>MCWAAAIPIAISGAQAISGQNAQAKMIAAQTAAGRRQAMEIMRQTNIQNADLSLQARSKLEEASAELTSQNMQKVQAIGSIRAAIGESMLEGSSMDRIKRVTEGQFIREANMVTENYRRDYQAIFAQQLGGTQSAASQIDEIYKSEQKQKSKLQMVLDPLAIMGSSAASAYASGAFDSKSTTKAPIVAAKGTKTGR[6x];>MRSYDMNVETAAELSAVNDILASIGEPPVSTLEGDANADAANARRILNKINRQIQSRGWTFNIEEGITLLPDVYSNLIVYSDDYLSLMSTSGQSIYVNRGGYVYDRTSQSDRFDSGITVNIIRLRDYDEMPECFRYWIVTKASRQFNNRFFGAPEVEGVLQEEEDEARRLCMEYEMDYGGYNMLDGDAFTSGLLTR[12x];>[18x]MANVIKTVLTYQLDGSNRDFNIPFEYLARKFVVVTLIGVDRKVLTINTDYRFATRTTISLTKAWGPADGYTTIELRRVTSTTDRLVDFTDGSILRAYDLNVAQIQTMHVAEEARDLTTDTIGVNNDGHLDARGRRIVNLANAVDDRDAVPFGQLKTMNQNSWQARNEALQFRNEAETFRNQAEGFKNESSTNATNTKQWRDETKGFRDEAKRFKNTAGQYATSAGNSASAAHQSEVNAENSATASANSAHLAEQQADRAEREADKLENYNGLAGAIDKVDGTNVYWKGNIHANGRLYMTTNGFDCGQYQQFFGGVTNRYSVMEWGDENGWLMYVQRREWTTAIGGNIQLVVNGQIITQGGAMTGQLKLQNGHVLQLESASDKAHYILSKDGNRNNWYIGRGSDNNNDCTFHSYVHGTTLTLKQDYAVVNKHFHVGQAVVATDGNIQGTKWGGKWLDAYLRDSFVAKSKAWTQVWSGSAGGGVSVTVSQDLRFRNIWIKCANNSWNFFRTGPDGIYFIASDGGWLRFQIHSNGLGFKNIADSRSVPNAIMVENE;>MALISQSIKNLKGGISQQPDILRYPDQGSRQVNGWSSETEGLQKRPPLVFLNTLGDNGALGQAPYIHLINRDEHEQYYAVFTGSGIRVFDLSGNEKQVRYPNGSNYIKTANPRNDLRMVTVADYTFIVNRNVVAQKNTKSVNLPNYNPNQDGLINVRGGQYGRELIVHINGKDVAKYKIPDGSQPEHVNNTDAQWLAEELAKQMRTNLSDWTVNVGQGFIHVTAPSGQQIDSFTTKDGYADQLINPVTHYAQSFSKLPPNAPNGYMVKIVGDASKSADQYYVRYDAERKVWTETLGWNTEDQVLWETMPHALVRAADGNFDFKWLEWSPKSCGDVDTNPWPSFVGSSINDVFFFRNRLGFLSGENIILSRTAKYFNFYPASIANLSDDDPIDVAVSTNRIAILKYAVPFSEELLIWSDEAQFVLTASGTLTSKSVELNLTTQFDVQDRARPFGIGRNVYFASPRSSFTSIHRYYAVQDVSSVKNAEDITSHVPNYIPNGVFSICGSGTENFCSVLSHGDPSKIFMYKFLYLNEELRQQSWSHWDFGENVQVLACQSISSDMYVILRNEFNTFLARISFTKNAIDLQGEPYRAFMDMKIRYTIPSGTYNDDTFTTSIHIPTIYGANFGRGKITVLEPDGKITVFEQPTAGWNSDPWLRLSGNLEGRMVYIGFNINFVYEFSKFLIKQTADDGSTSTEDIGRLQLRRA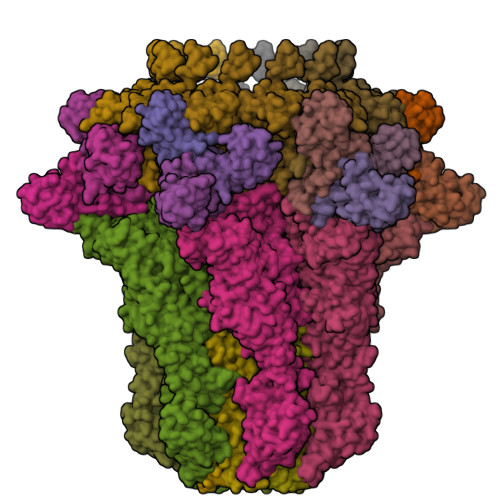WVNYENSGTFDIYVENQSSNWKYTMAGARLGSNTLRAGRLNLGTGQYRFPVVGNAKFNTVYILSDETTPLNIIGCGWEGNYLRRSSGI[6x]> SLGPPYHVIIDTNFINFCLQQKIDLFEGLMTCLYAKTIPCISDCVMAELEKLGIRYRIALRIAKDERFERLPCTHKGTYADDCIVQRVMQHKCYLVATNDKNLKQRIRKIPGIP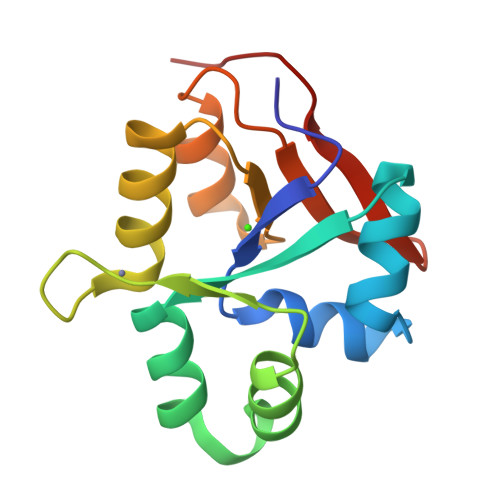ILSVANHKIRVERLVDVVD> MDQAANAAESATKDQLTQ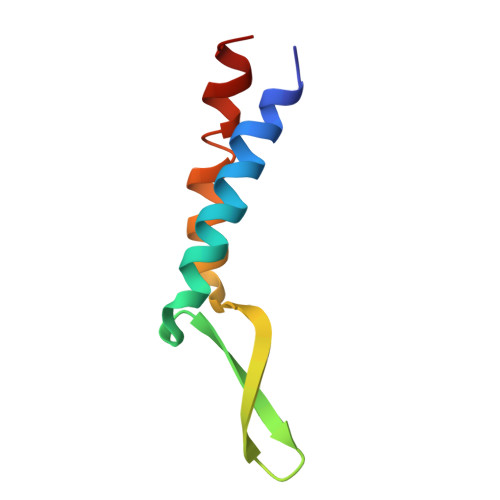EAFKNPENQKVNIDANGNAIPSGELKDDIVEQIAQQAKEAGEVARQQA>[3x]MHYAEAATPAKSAGSAVAKKHLEAKQKIGFVHGIDGTIATIAPAASKVTVPYNTVLEIAVSATNIANALVFNLEKDGSIGVILLDNISEVRSGQDVYATGSLLKIPVGFHMLGKIINPLGKEIPTGLFTKAAPLLDDTKLGLVEEMAPNIVSRQPVNYNLLTGYKVIDTLIPVGRGQRELILGDRQTGKTSIALSTILNQTKVNNEILSKNNVLSVYVSIGQRCSNVARIHRLLTEYDAMKYCTIVAATAADPAGLQYLAPYAGTTLGEEFRNSGRHILLVYDDLSKQAVSYRQISLLLRRPPGREAYPGDVFYLHSRLLERSAMMSPQKGSGSLTSLPIVETLSNDVTAYIVTNVISITDGQIYLDAKLFTGGQRPAVNIGLSVSRVGSSAQNKAMKKVGGALKMLMGEYRKMAGEQTSGSQNVSPVMIRGARCLQLFNQKGPSYFMDAIVALYAVTNGYMDDVKLQYSKFYEFLLLNKDLPVLYGQVNNKYFYMYNKNLNYFIRYFGLNHEILEPELKKYIEIHTNLFLDNYQSRMNELKSDEDLVQLKNLLYACKRTV;>[3x]TAPATAADVKQVGYVQQIIGAVVDVTFTDSVPPVLTALTVDAKETGTLLTMEIVQHLDTKTARCICMSSTDMLRLRTPVVNTGSQITVPVGEATLGRIFNVMGDAIDQRGPVKNKVRWPIHRKAPTLAEQSGKDEVLVTGIKVIDLILPYCKGGKIGLFGGAGVGKTVIIMELINNVAKGHGGYSVFAGVGERTREG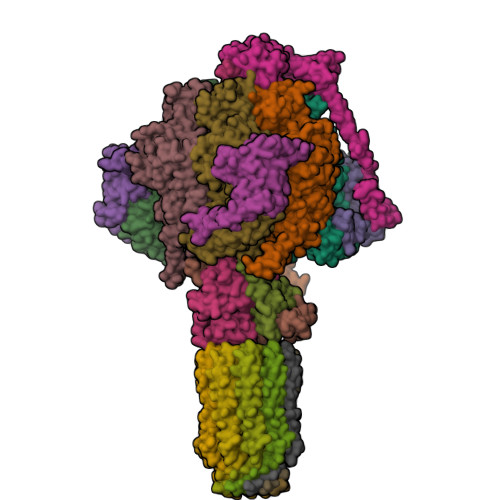TDLYLEMMGSKVIDLQGDSKCVLVYGQMNEPPGARARVAQTALTMAEYFRDEAGQDVLLFVDNVFRFTQANSEVSALLGRIPAAVGYQPTLAEDLGMLQERITSTVKGSITSVQAVYVPADDITDPAPATTFSHLDATTVLSRSVAEAGIYPAVEPLECASRIMDPDAIDVNHYNVAMDIVEMLTKYKELQDIIAVLGIDELSEEDKLIVDRARKVAKFMSQPFAVAEVFTGMKGYYVQLEDCVSDFGSLLMGQCDNIPEMAFYMVGGLDSVKEKAAKMAAEAAAMRERARKAAEAK;> MPGGGTIRFWREKLEGYKKYHQIVKTIKMVTLAKYRQTVVRTRVRDQTLRYTRKALDAKTQDDQEVIEKSECLLYVPITTNRGSCGALNTNMVRYLQEVENPKMTIISVGKKALDAMTKVFQDTYRRTILNDMKQAMSFQFAAYVLEHMNTVPWDRAQIVYNRYHGAASQKLAIFNLPKFEDWKQKLEEDSAGDGKIEEDGLLQSLPMKTALGELEETAVEDFYNFHSCLAVLNAVSENELSEYAARIVAVENQLGNITGLMQLADYTYNKTRKELITAELLEIIGTMTAMHAGKKVGLKKTEFWK;> MRASRTLLLSVSRFMRQDPRKFFPDNGFRFFDGPEDSFGDGNIPAQIILTLTRQDEFILKQEPVAAITIRTNEGEMGVLAGHEYTVQQLAPGILEVEYEGGKKDQYVISGGFAHVNDTGVVDINTVEAVPLEEIDHEKLAKALEEARAKSQSPDEAVRIQGEIALEIFEPLEAALH;> MSWRDAGISYLRYLSIVTRCIHEVQKEGPLLTKNVRFSTIGWKSLYLDHGATKEYTAIPAELEKIPENQVAQQHHA;>[3x]MQKLSRVVCNRLVRFHGTVAASAGGKRYDLFGYEVSVATGPFIEEIKKAQFYDDAGEVIVKMNLANTPPDLQTYNAVLERILNCKSKRSQPVKGENKFAAMMDILEEMDARSGIKPNAESWGYVLKELVQAGDFRLGWVCIAGMKSLGITPDQALVDANEANAAKAKAAGTDFPAYLKKAAPESFDTKAWGI;> MHMRRAVSVFGRCRSLNGLRNYAVPSPKYIEIYQSDFSRNAYPLELLGGSHVDFAKLLYSFADQVENKKFEVYVEDFKKLDSIIAEKGPFWAEEKIFQSPTFQGLSEGFKFILGWIQSEGAIDRLENVRLAYKELVNEARKETTATVIVAKEPSGNDLAEIRKQVEELHKESPLKDYKLVLETKVDPSIGGGYILEVCNQVVNRSAAAAAAETAALAKASAAQVDWTSLPAAPPRPSPSAPDTLIRLLGSVVDDLADADKVEQKYGA;>MQRGSSITKVVRRAALARSTRNAAIAYEVTVNGANLIGAGMAASGVGVPAIGVAMCFSSYMLAAARQPNMSAKLLPYCILGFALSEALALFTLLIALLELFVFS[10x]> GYTYEDYQDTAKWLLSHTEQRPQVAVICGSGLGGLVNKLTQAQTFDYSEIPNFPESTVPGHAGRLVFGILNGRACVMMQGRFHMYEGYPFWKVTFPVRVFRLLGVETLVVTNAAGGLNPNFEVGDIMLIRDHINLPGFSGQNPLRGPNEERFGVRFPAMSDAYDRDMRQKAHST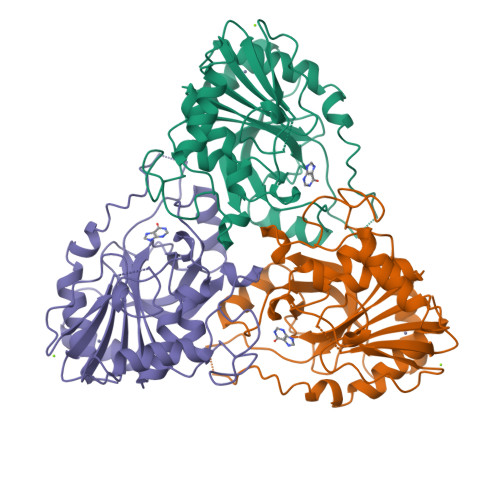WKQMGEQRELQEGTYVMLGGPNFETVAECRLLRNLGADAVGMSTVPEVIVARHCGLRVFGFSLITNKVIMDYESQGKANHEEVLEAGKQAAQKLEQFVSLLMASIPV>MGVVPQYGGGGNHGGGGNNSGPNSELNIYQYGGGNSALALQTDCRNSDLTITQHGGGNGADVGQGSDDSSIDLTQRGFGNSATLDQWNGKNSEMTVKQFGGGNGAAVDQTASNSS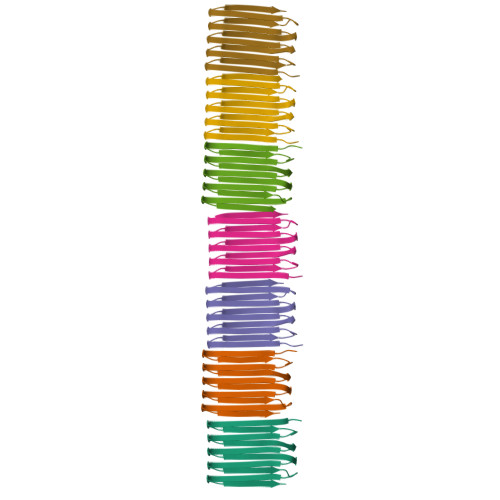VNVTQCGFGNNATAHQYHHHHHH[7x]>[2x]MGSEVYQSQKCELKYSKSQIEKAARKIRHGCEGAEREEAIKMIQNFRELHLYPLMLMKNHLDRAAKKVDKENKIIVARRLKRLSTIIDKLERPSLDGGATNNAIALTRMQDIGGCRAIVRNIEQLKKLKDRLVKSRSKHKILKEYDYLTPKPSGYSGIHLAYSCFDEENGNNPWSKTKIEVQLRTELQHAWATSLEIIDTLENIKLKTSNEGHPEWRRFFYLSGCLVAHDEGACILDDETIKNYQTELKTLEEALSVRSKLSTYTFAMKLTSDANLKKSLPKNHNGFFLVRMRNAITKNGKDTGKFLVSVKPFRKKESEQALQELNKDDADPEVLIAVLLATNNIKSLKKAYPNYFGSTNQFGRFLSRHIDTV

Here we identify and investigate the anti-phage function of CapRelSJ46, a fused toxin–antitoxin system that protects Escherichia coli against diverse phages. Using genetic, biochemical and structural analyses, we demonstrate that the C-terminal domain of CapRelSJ46 regulates the toxic N-terminal region, serving as both antitoxin and phage infection sensor. Following infection by certain phages, newly synthesized major capsid protein binds directly to the C-terminal domain of CapRelSJ46 to relieve autoinhibition, enabling the toxin domain to pyrophosphorylate tRNAs, which blocks translation to restrict viral infection. Collectively, our results reveal the molecular mechanism by which a bacterial immune system directly senses a conserved, essential component of phages, suggesting a PAMP-like sensing model for toxin–antitoxin-mediated innate immunity in bacteria.

To further understand the mechanistic basis of anti-phage defence by CapRelSJ46, we solved a crystal structure to 2.3 Å resolution. CapRelSJ46 contains a conserved, N-terminal nucleotide pyrophosphokinase domain (toxSYNTH) that is also present in alarmone synthetases and tRNA-pyrophosphotransferase enzymes, which mediates toxicity. The smaller C-terminal antitoxin domain consists of a central antiparallel three-stranded β-sheet with an α-helix connecting β-strands β7 and β8. The antitoxin domain is topologically analogous to the classical zinc-finger domain (ZFD), but lacks the conserved cysteines; we refer to this domain as a pseudo-ZFD. The pseudo-ZFD is connected to the toxSYNTH domain via α-helices α7, α8 and α9, and has a C-terminal α-helical extension that anchors the domain to α8 and α9. In this structure, the toxSYNTH and pseudo-ZFD are distant from each other, revealing the ATP donor nucleotide binding pocket and the conserved G-loop Y155 of toxSYNTH, indicating that this state may represent the active, toxic conformation of CapRelSJ46. This open state captured by crystallography is probably stabilized by crystal lattice contacts that are incompatible with a closing of the active site owing to clashes with symmetry-related partners. In addition to predicting the open conformation observed in the crystal structure, AlphaFold also predicted a closed conformational state in which the C-terminal domain folds back 110° onto the toxSYNTH central β-sheet and blocks the ATP-binding site. The crystal structure of CapRelSJ46 suggested that L280 and L307 in the wild-type protein promote the open, active state, with L280 stabilizing one of the hinge regions involving the pseudo-ZFD and L307 structuring the β6–β7 loop that interacts with Gp57 A-domain. Collectively, our results indicate that the pseudo-ZFD docks onto the ATP-binding site of CapRelSJ46 to prevent switching to the open state captured in our crystal structure.>[4x]AMGSMK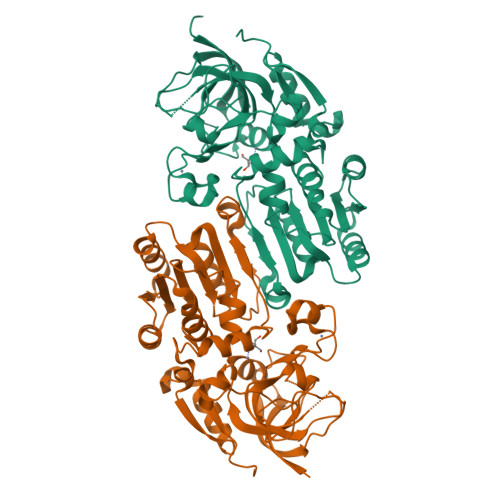AYTYVKPGLASFVDVDKPVIRKPTDAIVRIVKTTICGTDLHIIKGDVPTCQSGTILGHEGIGIVEEVGEGVSNFKKGDKVLISCVCACGKCYYCKKGIYAHCEDEGGWIFGHLIDGMQAEYLRVPHADNTLYHTPEDLSDEALVMLSDILPTGYEIGVLKGKVEPGCSVAIIGSGPVGLAALLTAQFYSPAKLIMVDLDDNRLETALSFGATHKVNSSDPEKAIKEIYDLTDGRGVDVAIEAVGIPATFDFCQKIIGVDGTVANCGVHGKPVEFDLDKLWIRNINVTTGLVSTNTTPQLLKALESHKIEPEKLVTHYFKLSEIEKAYEVFSKAADHHAIKVIIENDISEA> MKLSRISAINWNKISDDKDLEVWNRLTSNFWLPEKVPLSNDIPAWQTLTVVEQQLTMRVFTGLTLLDTLQNVIGAPSLMPDALTPHEEAVLSNISFMEAVHARSYSSIFSTLCQTKDVDAAYAWSEENAPLQRKAQIIQQHYRGDDPLKKKIASVFLESFLFYSGFWLPMYFSSRGKLTNTADLIRLIIRDEAVHGYYIGYKYQKNMEKISLGQREELKSFAFDLLLELYDNELQYTDELYAETPWADDVKAFLCYNANKALMNLGYEPLFPAEMAEVNPAILAALSPNADENHDFFSGSGSSYVMGKAV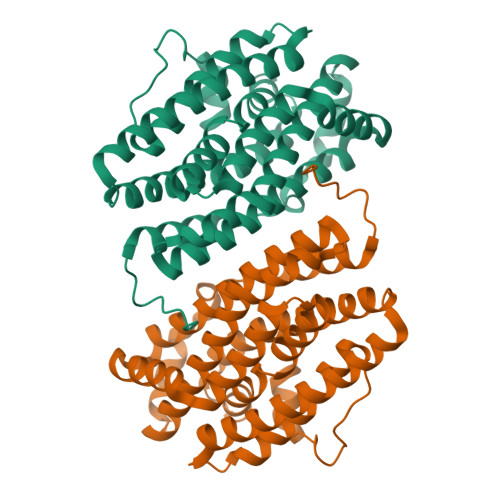ETEDEDWNF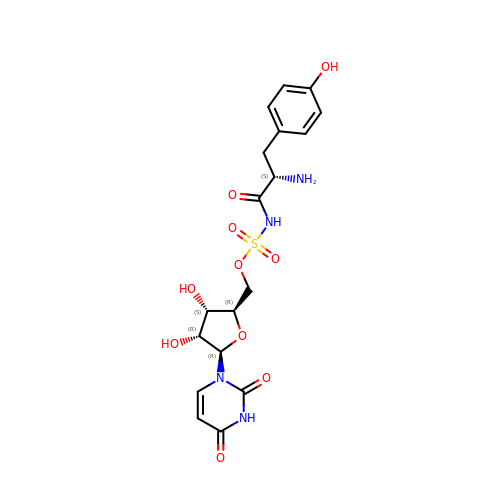[(2~{R},3~{S},4~{R},5~{R})-5-[2,4-bis(oxidanylidene)pyrimidin-1-yl]-3,4-bis(oxidanyl)oxolan-2-yl]methyl ~{N}-[(2~{S})-2-azanyl-3-(4-hydroxyphenyl)propanoyl]sulfamate | C18 H22 N4 O10 S | WEMPOZWVESAOCV-LMWHNAIISA-N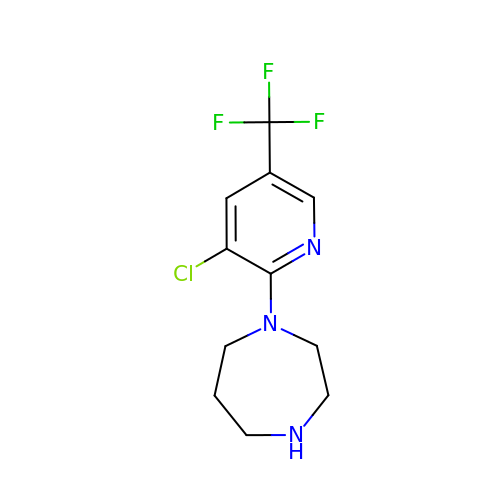1-[3-chloranyl-5-(trifluoromethyl)pyridin-2-yl]-1,4-diazepane | C11 H13 Cl F3 N3 | PKKLERQDFWUWNM-UHFFFAOYSA-N> SNARDPRPLRDKNFQSAIQEEIYDYLKKNKFDIETNHPISIKFLKQPTQKGFIIIFKWLYLRLDPGYGFTKSIENEIYQILKNLRYPFLESINKSQISAVGGSNWHKFLGMLHWMVRTNIKLDMCLNKVDRSLINQNTQEITILSQPL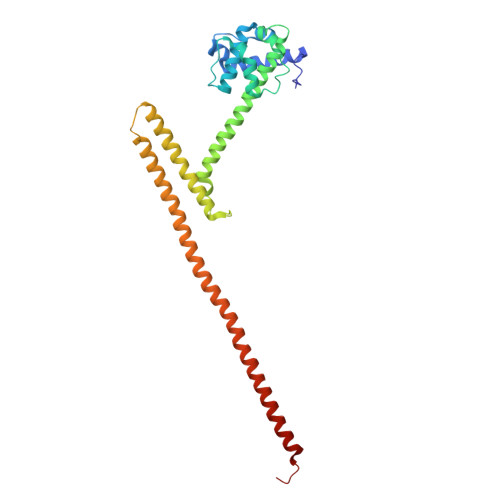KTLDEQDQRQERYELMVEKLLIDYFTESYKSFLKLEDNYEPSMQELKLGFEKFVHIINTDVTSTELKLEELKVDLNRKRYKLHQQVIHVIDITSKFKINIQSSLENSENELGNVIEELRNLEFE2-methylbenzoic 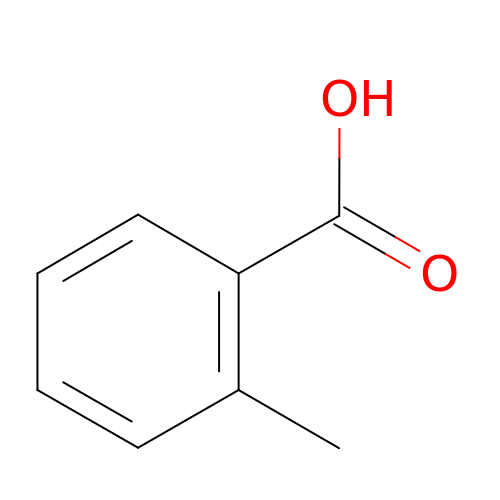acid | C8 H8 O2 | ZWLPBLYKEWSWPD-UHFFFAOYSA-N>[4x]MYEWKLNEIVDSGVCARCGTCTIVCPNGILTFDERPKLIDECLRKGHGMCFEVCPRVSSAKYQIKIREKFYEKYYYAKSDIEGQDGGVVTAFLKYLLENGKIDGAIVVGDECWKPVSLVVQNAEDLLKTAKSKYAISTLDALRKAGEMGLEKVAVVGLPCQINGLRKLQYFPYHAKHDLELGRNGKPVKLPKIEYLIGLFCTEKFRYDNMKEVLSKHGIDIEKVEKFDIKKGKLLVYVNGEKKEFDLKEFEICSGCKMCRDFDAEMADVSVGCVGSPDGYSTIIIRTEKGEEIKNAVELKEGVNLEEIEKLRQLKLKRFKKEVERRRENNEYVSFYWTADYGGIGKRADGTY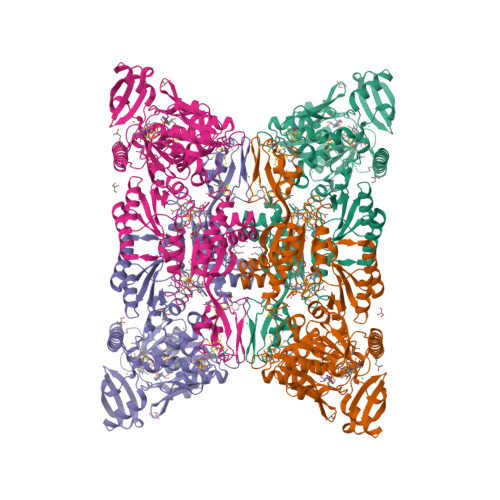FIRVRAKPGGWYKPEEIKEILDIAEEYNAKIKVTDRAGYELHGISGFDVEDIVLRLREKGLLTGSEGPLVRATLACPGGGNCSSGLVDTTELARIIEDNFKERPAPYKFKIAISGCPNGCVRPQVHDIGIAGVKYPKVNEEKCNGCGRCAEVCKVEAIDIRGETSYTNYNVCVGCGKCIKNCPNEAREVKEEGYLVYVGGKTGREVVEGVKMKLMSVDEIINFIDKVLVVYGKYAEKPQRERLAAVMKRVGYGKFLEEVKELMKKEIC> APAVAHHHHHHAVADKADNAFMMICTALVLFMTIPGIALFYGGLIRGKNVLSMLTQVTVTFALVCILWVVYGYSLAFGEGNNFFGNINWLMLKNIELTAVMGSIYQYIHVAFQGSFACITVGLIVGALAERIRFSAVLIFVVVWLTLSYIP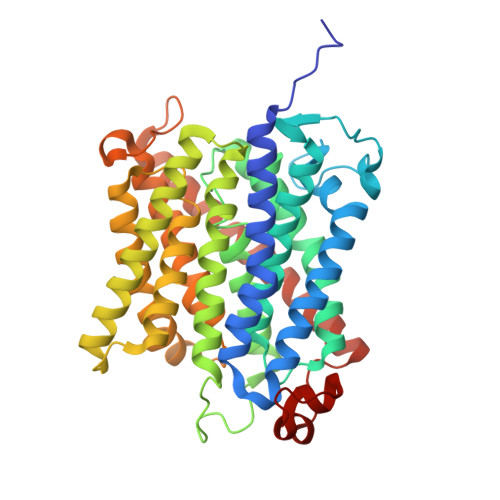IAHMVWGGGLLASHGALDFAGGTVVHINAAIAGLVGAYLIGKRVGFGKEAFKPHNLPMVFTGTAILYIGWFGFNAGSAGTANEIAALAFVNTVVATAAAILGWIFGEWALRGKPSLLGACSGAIAGLVGVTPACGYIGVGGALIIGVVAGLAGLWGVTMLKRLLRVDDPCDVFGVHGVCGIVGCIMTGIFAASSLGGVGFAEGVTMGHQLLVQLESIAITIVWSGVVAFIGYKLADLTVGLRVPEEQEREGLDVNSHGENAYNA> SEFGHRTLASTPALWASIPCPRSELRLDLVLPSGQSFRWREQSPAHWSGVLADQVWTLTQTEEQLHCTVYRGDKSQASRPTPDELEAVRKYFQLDVTLAQLYHHWGSVDSHFQEVAQKFQGVRLLRQDPIECLFSFICSSCNNIARITGMVERLCQAFGPRLIQLDDVTYHGFPSLQ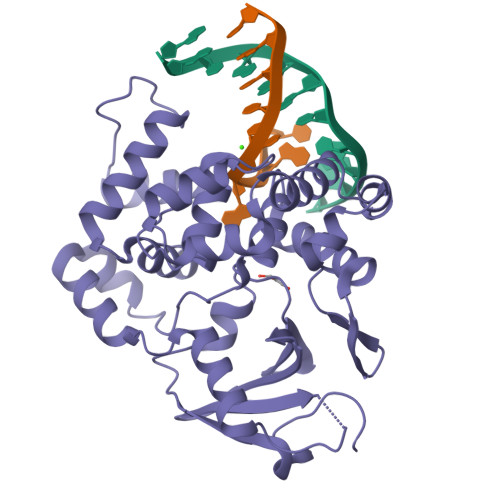ALAGPEVEAHLRKLGLGYRARYVSASARAILEEQGGLAWLQQLRESSYEEAHKALCILPGVGTKVADCICLMALDKPQAVPVDVHMWHIAQRDYSWHPTTSQAKGPSPQTNKELGNFFRSLWGPYAGWAQAVLFSADLRQSR> SEISRQEFQRRRQALVEQMQPGSAALIFAAPEV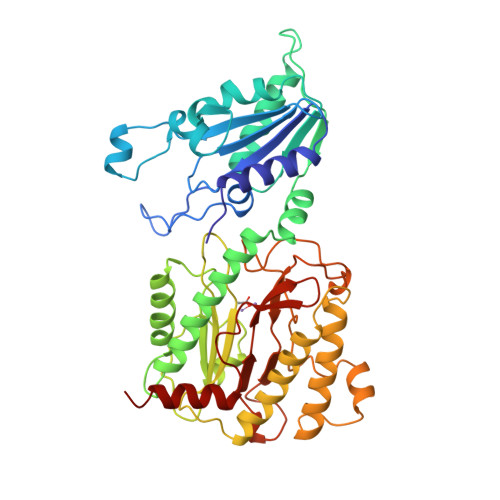TRSADSEYPYRQNSDFWYFTGFNEPEAVLVLIKSDDTHNHSVLFNRVRDLTAEIWYGRRLGQDAAPEKLGVDRALAFSEINQQLYQLLNGLDVVYHAQGEYAYADVIVNSALEKLRKGSRQNLTAPATMIDWRPVVHEMRLFKSPEEIAVLRRAGEITAMAHTRAMEKCRPGMFEYHLEGEIHHEFNRHGARYPSYNTIVGSGENGCILHYTENECEMRDGDLVLIDAGCEYKGYAGDITRTFPVNGKFTQAQREIYDIVLESLETSLRLYRPGTSILEVTGEVVRIMVSGLVKLGILKGDVDELIAQNAHRPFFMHGLSHWLGLDVHDVGVYGQDRSRILEPGMVLTVEPGLYIAPDAEVPEQYRGIGIRIEDDIVITETGNENLTASVVKKPEEIEALMVAARKQ> GPGSMGVPICGACRRPIEGRVVNAMGKQWHVEHFVCAKCEKPFLGHRHYERK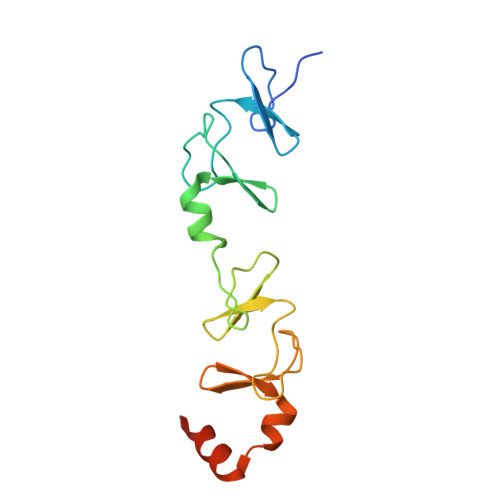GLAYCETHYNQLFGDVCFHCNRVIEGDVVSALNKAWCVNCFACSTCNTKLTLKNKFVEFDMKPVCKKCYEKFPLELKKRLKKLAETLGRK[[(2~{R},3~{S},4~{R},5~{R})-5-(3-aminocarbonyl-4~{H}-pyridin-1-yl)-3,4-bis(oxidanyl)oxolan-2-yl]methoxy-oxidanyl-phosphoryl] 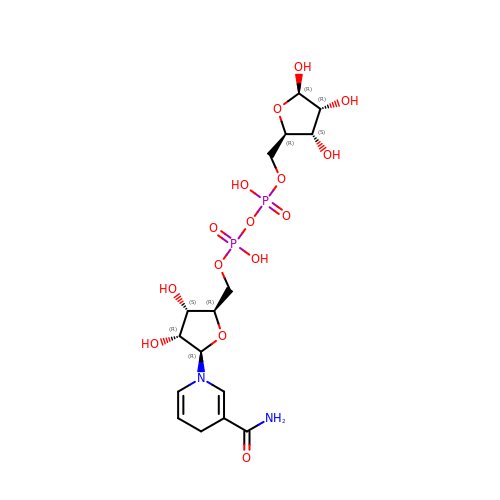[(2~{R},3~{S},4~{R},5~{R})-3,4,5-tris(oxidanyl)oxolan-2-yl]methyl hydrogen phosphate | C16 H26 N2 O15 P2 | CORMEBAPIXUNEL-UDOSWUQBSA-N> MKDLLKFLKAQTKTEEFDAIKIALASPDMIRSWSFGEVKKPETINYRTFKPERDGLFCARIFGPVKDYECLCGKYKRLKHRGVICEKCGVEVTQTKVRRERMGHIELASPTAHIWFLKSLPSRIGLLLDMPLRDIERVLYFESYVVIEGGMTNLERQQILTEEQYLDALEEFGDEFDAKMGAEAIQALLKSMDLEQECEQLREELNETNSETKRKKLTKRIKLLEAFVQSGNKPEWMILTVLPVLPPDLRPLVPLDGGRFATSDLNDLYRRVINRNNRLKRLLDLAAPDIIVRNEKRMLQEAVDALLDNGRRGRAITGSNKRPLKSLADMIKGKQGRFRQNLLGKRVDYSGRSVITVGPYLRLHQCGLPKKMALELFKPFIYGKLELRGLATTIKAAKKMVEREEAVVWDILDEVIREHPVLLNRAPTLHRLGIQAFEPVLIEGKAIQLHPLVCAAYNADFDGDQMAVHVPLTLEAQLEARALMMSTNNILSPANGEPIIVPSQDVVLGLYYMTRDCVNAKGEGMVLTGPKEAERLYRSGLASLHARVKVRITEYEKDANGELVAKTSLKDTTVGRAILWMIVPKGLPYSIVNQALGKKAISKMLNTCYRILGLKPTVIFADQIMYTGFAYAARSGASVGIDDMVIPEKKHEIISEAEAEVAEIQEQFQSGLVTAGERYNKVIDIWAAANDRVSKAMMDNLQTETVINRDGQEEKQVSFNSIYMMADSGARGSAAQIRQLAGMRGLMAKPDGSIIETPITANFREGLNVLQYFISTHGARKGLADTALKTANSGYLTRRLVDVAQDLVVTEDDCGTHEGIMMTPVIEGGDVKEPLRDRVLGRVTAEDVLKPGTADILVPRNTLLHEQWCDLLEENSVDAVKVRSVVSCDTDFGVCAHCYGRDLARGHIINKGEAIGVIAAQSIGEPGTQLTMRTFHIGGAASRAAAESSIQVKNKGSIKLSNVKSVVNSSGKLVITSRNTELKLIDEFGRTKESYKVPYGAVLAKGDGEQVAGGETVANWDPHTMPVITEVSGFVRFTDMIDGQTITRQTDELTGLSSLVVLDSAERTAGGKDLRPALKIVDAQGNDVLIPGTDMPAQYFLPGKAIVQLEDGVQISSGDTLARIPQESGGTKDITGGLPRVADLFEARRPKEPAILAEISGIVSFGKETKGKRRLVITPVDGSDPYEEMIP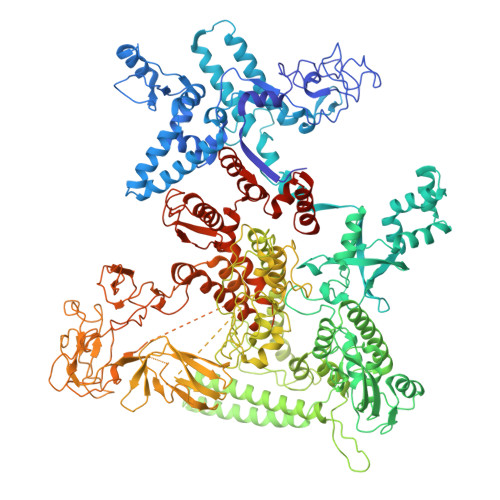KWRQLNVFEGERVERGDVISDGPEAPHDILRLRGVHAVTRYIVNEVQDVYRLQGVKINDKHIEVIVRQMLRKATIVNAGSSDFLEGEQVEYSRVKIANRELEANGKVGATYSRDLLGITKASLATESFISAASFQETTRVLTEAAVAGKRDELRGLKENVIVGRLIPAGTGYAYHQDRMRRRAAGEAPAAPQVTAEDASASLAELLNAGLGGSDN> GSHMPLSSENKQKLQKQVEFYFSDVNVQRDIFLKGKMAENAEGFVSLETLLTFKRVNSVTTDVKEVV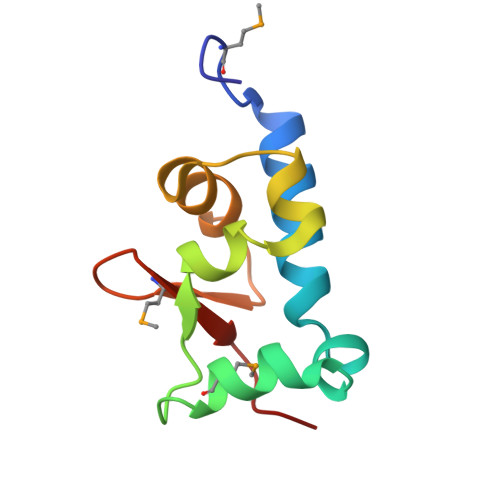EAIRPSEKLVLSEDGLMVRRRDPLP> CGGRARVREYSRAELVIGTLCRVRVYSKRPAAEVHAALEEVFTLLQQQEMVLSANRDDSALAALNAQAGSAPVVVDRSLYALLERALFFAEKSGGAFNPALGAVVKLWNIGFDRAAVPDPDALKEALTRCDFRQVHLRAGVSVGAPHTVQLAQAGMQLDLGAIAKGFLADKIVQLLTAHALDSALVDLGGNIFALGLKYGDVRSAAAQRLEWNVGIRDPHGTGQKPALVVSVRDCSVVTSGAYERFFERDGVRYHHIIDP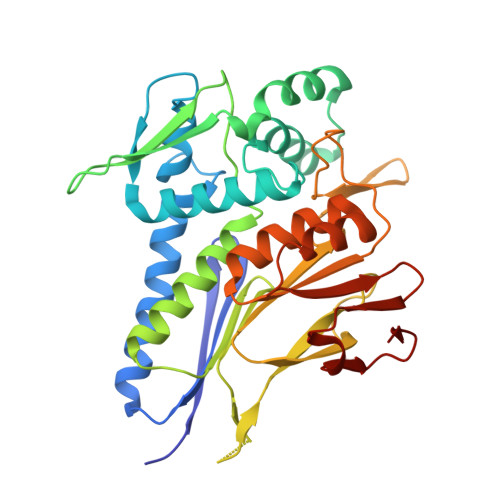VTGFPAHTDVDSVSIFAPRSTDADALATACFVLGYEKSCALLREFPGVDALFIFPDKRVRASAGIVDRVRVLDARFVLER> 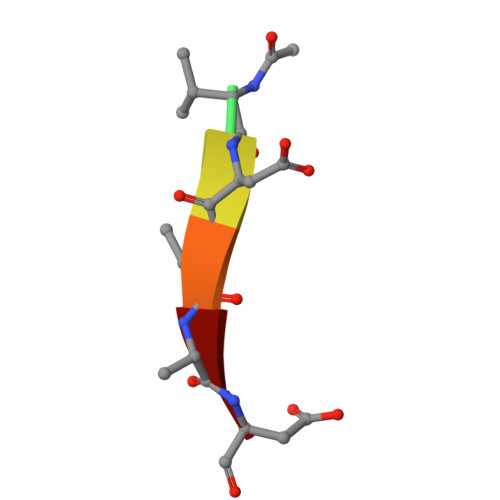XVDVAD> GPMTSATAHETVATGEGLRQALVGQPASLTVTTKDKDGRLVRTGSAELRAEITGPDGTRLPVPVVDHKNGTYELVYTARTEGELLLSVL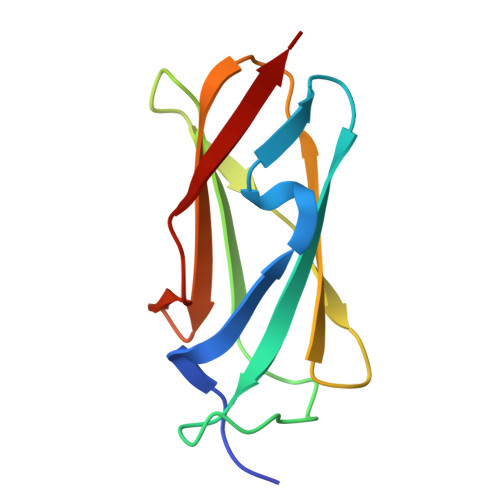LYGQPVRGSPFRVRALR> MNDQPFAWQVASLSERYQEQFDIGAAVEPYQLEGRQAQILKHHYNSLVAENAMKPESLQPREGEWNWEGADKIVEFARKHNMELRFHTLVWHEQVPEWFFIDEDGNRMVDETDPDKREANKQLLLERMENHIKTVVERYKDDVTSWDVVNEVIDDGGGLRESEWYQITGTDYIKVAFETARKYGGEEAKLYINDYNTEVPSKRDDLYNL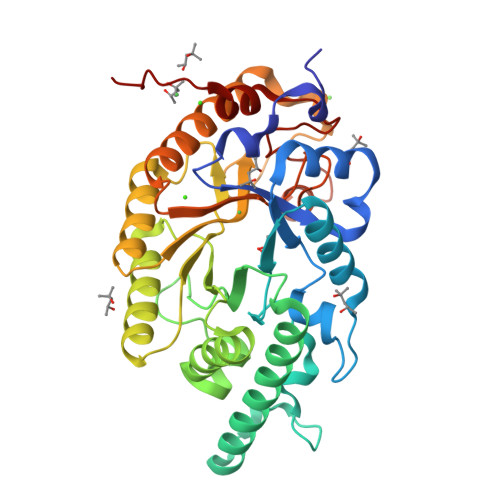VKDLLEQGVPIDGVGHQSHIQIGWPSIEDTRASFEKFTSLGLDNQVTELDMSLYGWPPTGAYTSYDDIPAELLQAQADRYDQLFELYEELAADISSVTFWGIADNHTWLDGRAREYNNGVGIDAPFVFDHNYRVKPAYWRIIDLEHHHHHH>MPPTSVSPPRTAPGPANPSPAHPSRVRVIHPGGGKPGGPVVYWMLRDQRLADNWALLHAAGLAAASASPLAVAFALFPRPFLLSARRRQLGFLLRGLRRLAADAAARHLPFFLFTGGPAEIPALVQRLGASTLVADFSPLRPVREALDAVVGDLRREAPGVAVHQVDAHNVVPVWTASAKMEYSAKTFRGKVSKVMDEYLVEFPELPAVVPWDREQPEGVDWDALIARVCSEAENVPEIDWCEPGEEAAIEALLGSKDGFLTKRIKSYETDRNDPTKPRALSGLSPYLHFGHISAQRCALEAKKCRHLSPKSVDAFLEELVVRRELADNFCYYQPQYDSLSGAWEWARKTLMDHAADKREHIYTREQLENAKTHDPLWNASQLEMVHHGKMHGFMRMYWAKKILEWTSGPEEALSTAIYLNDKYEIDGRDPSGYVGC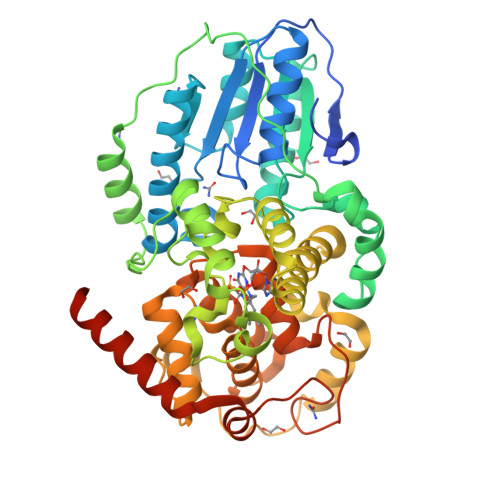MWSICGLHDQGWKERPVFGKIRYMNYAGCKRKFDVDAYISYVKRLAGQSKKRNAEESPNPVVKLSKSQH[2x]> GSERPKLDEGFYEIEAIRRKRVRKGKVQYLIKWRGWPETANTWEPLENLQSIADV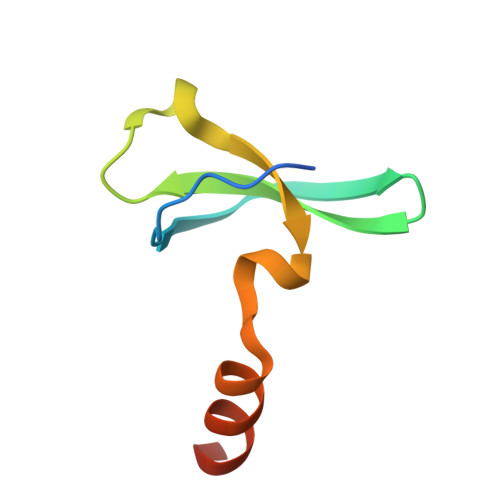IDAFEGSLKPG Transcription initiation in bacteria involves the recruitment of RNAP by sigma factors (σ) to promoter regions located upstream from the transcription start site (TSS, position +1). In approximately 60% of bacteria, a major variant σ factor, σ54, forms a class of its own, lacking structural and sequence similarity to σ70. In σ54-mediated transcription initiation, σ54 recruits RNAP to genes responsible for regulating a variety of stress responses, including nutrient depletion, membrane stress, antibiotic exposure, and biofilm formation. In this study, we used single-particle cryo-electron microscopy (cryoEM) to determine the structures of initial transcribing complexes of increasing RNA lengths from 5 nt to 9 nt, which allow us to propose a mechanism of RNAP promoter escape in the σ54 system.

Using a combination of focused classification and electron density subtraction, we obtained several distinct structural states within the same dataset, including pre- and post-translocated RNA states, as well as σ-free states. We focused on the pre- and post-translocated states which were resolved to 2.8 and 3.4 Å resolution respectively based on gold standard Fourier Shell Correlation curves. We could resolve almost the entire RNAP (including one α-CTD), DNA between −29 and +20, 5 nt RNA as well as σ54 CBD, ELH-HTH, and RpoN domains. In the RPitc-5nt structures, we could resolve extra residues in RII, including 93–106 (Inset). In RPitc-5nt, residues 104–112 form the tip of a β-hairpin (Inset), and residues 93–103 emerge from the β subunit side of the RNAP instead (Left). We now refer to this β-hairpin (residues 104–112) as the RII-finger due to its functional similarity with the σ70 finger, also known as R3.2 in σ70. In RPitc-5nt, RII contacts the template strand at the −5 position, and threads around the template DNA–RNA hybrid and forms a sharp kink at P110 (Inset). The RII-finger is stabilized by hydrophobic interactions between P110 and Y112 of RII, and the conserved P251, V253, and P254 on the β′ lid and M330 on β′ switch 2 region (Inset). During initial transcription, as in RPitc-5nt, the template strand expands into the back of the cleft. The template strand now interacts with the σ54 RII-finger.

>[2x]SVTEFLKPRLVDIEQVSSTHAKVTLEPLERGFGHTLGNALRRILLSSMPGCAVTEVEIDGVLHEYSTKEGVQEDILEILLNLKGLAVRVQGKDEVILTLNKSGIGPVTAADITHDGDVEIVKPQHVICHLTDENASISMRIKVQRGRGYVPASTRIHSEEDERPIGRLLVDACYSPVERIAYNVEAARVEQRTDLDKLVIEMETNGTIDPEEAIRRAATILAEQLEAFVDLRDVRQPEVKEEKPEFDPILLRPVDDLELTVRSANCLKAEAIHYIGDLVQRTEVELLKTPNLGKKSLTEIKDVLASRGLSLGMRLENWPPA;> MVYSYTEKKRIRKDFGKRPQVLDVPYLLSIQLDSFQKFIEQDPEGQYGLEAAFRSVFPIQSYSGNSELQYVSYRLGEPVFDVQECQIRGVTYSAPLRVKLRLVIYEREAPEGTVKDIKEQEVYMGEIPLMTDNGTFVINGTERVIVSQLHRSPGVFFDSDKGKTHSSGKVLYNARIIPYRGSWLDFEFDPKDNLFVRIDRRRKLPATIILRALNYTTEQILDLFFEKVIFEIRDNKLQMELVPERLRGETASFDIEANGKVYVEKGRRITARHIRQLEKDDVKLIEVPVEYIAGKVVAKDYIDESTGELICAANMELSLDLLAKLSQSGHKRIETLFTNDLDHGPYISETLRVDPTNDRLSALVEIYRMMRPGEPPTREAAESLFENLFFSEDRYDLSAVGRMKFNRSLLREEIEGSGILSKDDIIDVMKKLIDIRNGKGEVDDIDHLGNRRIRSVGEMAENQFRVGLVRVERAVKERLSLGDLDTLMPQDMINAKPISAAVKEFFGSSQLSQFMDQNNPLSEITHKRRISALGPGGLTRERAGFEVRDVHPTHYGRVCPIETPEGPNIGLINSLSVYAQTNEYGFLETPYRKVTDGVVTDEIHYLSAIEEGNYVIAQANSNLDEEGHFVEDLVTCRSKGESSLFSRDQVDYMDVSTQQVVSVGASLIPFLEHDDANRALMGANMQRQAVPTLRADKPLVGTGMERAVAVDSGVTAVAKRGGVVQYVDASRIVIKVNEDEMYPGEAGIDIYNLTKYTRSNQNTCINQMPCVSLGEPVERGDVLADGPSTDLGELALGQNMRVAFMPWNGYNFEDSILVSERVVQEDRFTTIHIQELACVSRDTKLGPEEITADIPNVGEAALSKLDESGIVYIGAEVTGGDILVGKVTPKGETQLTPEEKLLRAIFGEKASDVKDSSLRVPNGVSGTVIDVQVFTRDGVEKDKRALEIEEMQLKQAKKDLSEELQILEAGLFSRIRAVLVAGGVEAEKLDKLPRDRWLELGLTDEEKQNQLEQLAEQYDELKHEFEKKLEAKRRKITQGDDLAPGVLKIVKVYLAVKRRIQPGDKMAGRHGNKGVISKINPIEDMPYDENGTPVDIVLNPLGVPSRMNIGQILETHLGMAAKGIGDKINAMLKQQQEVAKLREFIQRAYDLGADVRQKVDLSTFSDEEVMRLAENLRKGMPIATPVFDGAKEAEIKELLKLGDLPTSGQIRLYDGRTGEQFERPVTVGYMYMLKLNHLVDDKMHARSTGSYSLVTQQPLGGKAQFGGQRFGEMEVWALEAYGAAYTLQEMLTVKSDDVNGRTKMYKNIVDGNHQMEPGMPESFNVLLKEIRSLGINIELED;> LLKFLKAQTKTEEFDAIKIALASPDMIRSWSFGEVKKPETINYRTFKPERDGLFCARIFGPVKDYECLCGKYKRLKHRGVICEKCGVEVTQTKVRRERMGHIELASPTAHIWFLKSLPSRIGLLLDMPLRDIERVLYFESYVVIEGGMTNLERQQILTEEQYLDALEEFGDEFDAKMGAEAIQALLKSMDLEQECEQLREELNETNSETKRKKLTKRIKLLEAFVQSGNKPEWMILTVLPVLPPDLRPLVPLDGGRFATSDLNDLYRRVINRNNRLKRLLDLAAPDIIVRNEKRMLQEAVDALLDNGRRGRAITGSNKRPLKSLADMIKGKQGRFRQNLLGKRVDYSGRSVITVGPYLRLHQCGLPKKMALELFKPFIYGKLELRGLATTIKAAKKMVEREEAVVWDILDEVIREHPVLLNRAPTLHRLGIQAFEPVLIEGKAIQLHPLVCAAYNADFDGDQMAVHVPLTLEAQLEARALMMSTNNILSPANGEPIIVPSQDVVLGLYYMTRDCVNAKGEGMVLTGPKEAERLYRSGLASLHARVKVRITEYEKDANGELVAKTSLKDTTVGRAILWMIVPKGLPYSIVNQALGKKAISKMLNTCYRILGLKPTVIFADQIMYTGFAYAARSGASVGIDDMVIPEKKHEIISEAEAEVAEIQEQFQSGLVTAGERYNKVIDIWAAANDRVSKAMMDNLQTETVINRDGQEEKQVSFNSIYMMADSGARGSAAQIRQLAGMRGLMAKPDGSIIETPITANFREGLNVLQYFISTHGARKGLADTALKTANSGYLTRRLVDVAQDLVVTEDDCGTHEGIMMTPVIEGGDVKEPLRDRVLGRVTAEDVLKPGTADILVPRNTLLHEQWCDLLEENSVDAVKVRSVVSCDTDFGVCAHCYGRDLARGHIINKGEAIGVIAAQSIGEPGTQLTMRTFHIGGAASRAAAESSIQVKNKGSIKLSNVKSVVNSSGKLVITSRNTELKLIDEFGRTKESYKVPYGAVLAKGDGEQVAGGETVANWDPHTMPVITEVSGFVRFTDMIDGQTITRQTDELTGLSSLVVLDSAERTAGGKDLRPALKIVDAQGNDVLIPGTDMPAQYFLPGKAIVQLEDGVQISSGDTLARIPQESGGTKDITGGLPRVADLFEARRPKEPAILAEISGIVSFGKETKGKRRLVITPVDGSDPYEEMIPKWRQLNVFEGERVERGDVISDGPEAPHDILRLRGVHAVTRYIVNEVQDVYRLQGVKINDKHIEVIVRQMLRKATIVNAGSSDFLEGEQVEYSRVKIANRELEANGKVGATYSRDLLGITKASLATESFISAASFQETTRVLTEAAVAGKRDELRGLKENVIVGRLIPAGTGYAYHQDRMRRRAAG;> ARVTVQDAVEKIGNRFDLVLVAARRARQMQVGGKDPLVPEENDKTTVIALREIEEGLINNQILDVRERQEQQEQ;> TAGTPSGNGVDYQDDELPVYQGETTQSLQDYLMWQVELTPFTDTDRAIATSIVDAVDDTGYLTIQIEDIVDSIGDDEIGLEEVEAVLKRIQRFDPVGVAAKDLRDCLLIQLSQFAKETPWLEEARLIISDHLDLLANHDFRTLMRVTRLKEEVLKEAVNLIQSLDPRPGQSIQTGEPEYVIPDVLVRKVNDRWVVELNSDSLPRLKINQQYAAMGNSARNDADGQFIRSNLQEARWLIKSLESANDTLLRVSRCIVEQQQAFFEQGEEYMKPMVLADIAQAVEMHESTISRVTTQKYLHSPRGIFELKYFFSSHVNTEGGGEASSTAIRALVKKLIAAENPAKPLSDSKLTSMLSEQGIMVARRTVAKYRESLSIPPSNQ Here, we report that some flavonoids act as the inhibitors of the Ae. aegypti Noppera-bo (AeNobo) protein, which belongs to the glutathione S-transferase (GST) epsilon subfamily. Nobo plays a specialized role in the biosynthesis of the principal insect steroid hormones, ecdysteroids. As ecdysteroids are particularly important for the life cycle of insects, it is expected that a chemical inhibitor of ecdysteroidogenic enzymes, including Nobo, would be an insect growth regulator (IGR) that impacts insect development without affecting organisms other than insects. AeNobo adopts a canonical GST fold, which has a well-conserved GSH-binding site (G-site) and a hydrophobic substrate-binding pocket (H-site) adjacent to the G-site.

We prepared a purified AeNobo recombinant protein (220-aa length) using an Escherichia coli protein expression system. Using this system, we found that the specific enzymatic activity of AeNobo to conjugate glutathione (GSH) and 3,4-DNADCF was 2.04 ± 0.04 μmol·min−1·mg−1 in vitro, suggesting that AeNobo exhibits GST enzymatic activity. To reveal the molecular mechanism through which these flavonoids inhibit AeNobo enzymatic activity, we conducted an X-ray crystallographic analysis of AeNobo. Gel filtration chromatography revealed that AeNobo forms a homodimer in solutions, suggesting that its dimeric structure is a biological unit similar to DmNobo and other canonical GSTs. We found that the asymmetric unit of AeNobo is composed of four chains: A, B, C, and D. Each chain forms a biological dimer with a symmetry-related subunit by a crystallographic twofold axis. The subunit structures of AeNobo complex with inhibitors were essentially the same as those of the substrate-free form. Interactions between AeNobo and GSH in the G-site were essentially the same in the presence or absence of daidzein or luteolin, suggesting that these flavonoids do not interfere with the interaction between AeNobo and GSH.

>MNHKVHMMSKPVLYYDDISPPVRGVLLTVAALGIKDQVELKLVRLFEREHLLEDFVKLNPLHAVPVLKHDDLVLTDSHAIIMYLCDIFGQDGDFSLKDPKQRARVHNRLCFNNAVLFQRESIVMRGLINRSIVTLEDHHLKPVQEAYDCLEVYLTNSKFVACDQLTVADFPIVACMSTVGMVCPLSTSRWPKTAAWFETMKQLPYYQQANQVGVDKLKERLHAVMKK[4x]> MDYHKILTAGLSVQQGIVRQRVIPVYQVNNLEEICQLIIQAFEAGVDFQESADSFLLMLCLHHAYQGDYKLFLESGAVKYLEGHGFRFEVKKRDGVKRLEELLPAVSSGKNIKRTLAAMPEEETTEANAGQFLSFASLFLPKLVVGEKACLEKVQ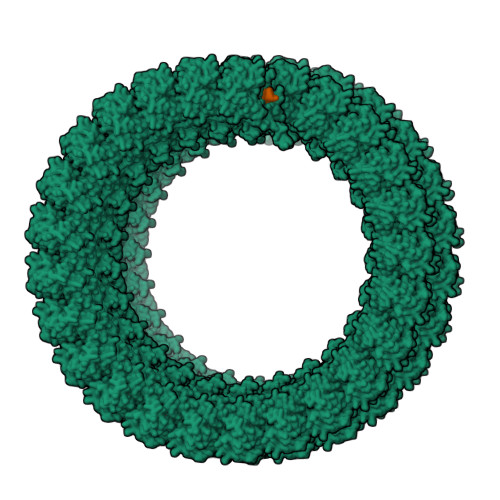RQIQVHAEQGLIQYPTAWQSVGHMMVIFRLMRTNFLIKFLLIHQGMHMVAGHDANDAVISNSVAQARFSGLLIVKTVLDHILQKTERGVRLHPLARTAKVKNEVNSFKAALSSLAKHGEYAPFARLLNLSGVNNLEHGLFPQLSAIALGVATAHGSTLAGVNVGEQYQQLREAATEAEKQLQQYAESRELDHLGLDDQEKKILMNFHQKKNEISFQQTNAMVTLRKERLAKLT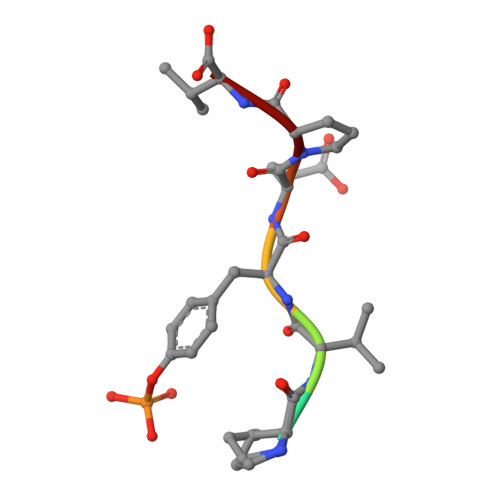> PPVYEPV> NLPDCDIDNWLNNVSVPSPLNWERRIFSNCNFNLSTLLRLVHVDSFSCNNLDKSKIFGSCFNSITVDKFAIPNRRRDDLQLGSSGFLQSSNYKIDISSSSCQLYYSLPLVNVTINNFNPSSWNRRYGFGSFNLSSYDVVYSDHCFSVNSDFCPCADPSVVNSCAKSKPPSAICPAGTKYRHCDLDTTLYVKNWCRCSCLPDPISTYSPNTCPQKKVVVGIGEHCPGLGINEEKCGTQLNHSSCFCSPDAFLGWSFDSCISNNRCNIFSNFIFNGINSGTTCSNDL;> MGSKCSNSGIECDSSGTCINPSNWCDGVSHCPGGEDENRCVRLYGPNFILQVYSSQRKSWHPVCQDDWNENYGRAACRDMGYKNNFYSSQGIVDDSGSTSFMKLNTSAGNVDIYKKLYHSDACSSKAVVSLRCIACGVNLNSSRQSRIVGGESALPGAWPWQVSLHVQNVHVCGGSIITPEWIVTAAHCVEKPLNNPWHWTAFAGILRQSFMFYGAGYQVEKVISHPNYDSKTKNNDIALMKLQKPLTFNDLVKPVCLPNPGMMLQPEQLCWISGWGATEEKGKTSEVLNAAKVLLIETQRCNSRYVYDNLITPAMICAGFLQGNVDSCQGDAGGPLVTSKNNIWWLIGDTSWGSGCAKAYRPGVYGNVMVFTDWIYRQMRADG

As a member of the Embecovirus, HKU1 uses a primary glycan-based receptor (9-O-acetylated sialosides) and a secondary proteinaceous receptor for host cell targeting and membrane fusion. One unique feature of HKU1 spike is that the C-terminal domain (CTD) of S1 (also known as receptor-binding domain, RBD) is exceptionally larger than other CoV RBDs, and the receptor-binding motif (RBM) of HKU1 adopts a unique fold. Proteinaceous receptor of HKU1 was identified as transmembrane serine protease 2 (TMPRSS2) and HKU1 RBD binds TMPRSS2 with nanomolar affinity. The TMPRSS2–RBD interaction occurred between a groove formed on the HKU1 RBD apex and a hydrophobic surface near the active site in the C-terminal trypsin-like serine peptidase (SP) domain of TMPRSS2.

Using bio-layer interferometry (BLI), we determined the equilibrium dissociation constant (KD) for RBD–TMPRSS2 interaction. The affinity of 1A-RBD–TMPRSS2 (KD = 323 nM) was ~2-fold lower than that of 1B-RBD–TMPRSS2 (KD = 170 nM), which is consistent with the KD values reported previously. The difference between 1A-RBD–TMPRSS2 and 1B-RBD–TMPRSS2 maps may attribute to higher binding affinity of 1B RBD for TMPRSS2 that enhances stability of the complex. Therefore, we mainly used 1B-RBD–TMPRSS2 structure for subsequent structural analysis. RBG is an arch-shaped module comprising an antiparallel β-hairpin (β10–β11, previously referred to as a horn) and a proline-rich loop; two disulfide bridges C504–C518 and C520–C533 stabilize the fold of this module. We identified 14 HKU1 spike residues and 8 TMPRSS2 residues mediating the interactions, rendering an interfacial area of 752 Å2. In particular, residues T509, L510, Y511, V512 and W515 on the β-hairpin of RBG are packed against a hydrophobic patch on TMPRSS2 formed by residues Y416, L419 and W461. Residues L521, P522, T527, Y528 and S529 from the proline-rich loop of RBG interact with a hydrophobic protrusion formed by L430, Y414 and Y469 of TMPRSS2. A π-stacking interaction is formed between TMRPSS2 R470 and 1B RBD R517. Additionally, the salt bridges between HKU1 spike D507 and TMPRSS2 R470, and between HKU1 spike D505 and TMPRSS2 K467 further stabilize the TMPRSS2–RBD interaction. Lastly, HKU1 spike K487 forms an additional salt bridge with TMPRSS2 D417, and this is the only non-RBG residue contributing to the interaction.> GSNQNTTEPVAATETLAEVPEHVLRGLPEEVRLFPSAVDKTRIGVWATKPILKGKKFGPFVGDKKKRSQVKNNVYMWEVYYPNLGWMCIDATDPEKG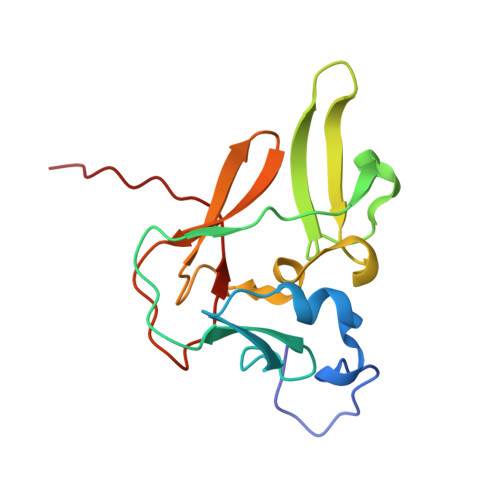NWLRYVNWACSGEEQNLFPLEINRAIYYKTLKPIAPGEELLVWYNGEDNPEI Heterogeneous nuclear ribonucleoprotein D0 (hnRNP D0), also known as AU-rich element RNA-binding protein 1 (AUF1), is a well-characterized ARE-binding factor that destabilizes mRNA, while human (Hu) antigen proteins of the ELAV (embryonic lethal, abnormal vision) family are known to stabilize mRNA. AUF1 has four isoforms, p37, p40, p42, and p45, generated by alternative splicing. AUF1 contains two tandem RRMs and an adjacent Q-rich motif. Many proteins regulate mRNA stability by interacting with the AU-rich elements (AREs) in the 3′-untranslated regions (3′-UTRs) of mRNAs.

We obtained the AUF1-p37RRMs protein by RNase treatment and determined the high resolution crystal structure of AUF1-RRM1. A selected AUF1-p37RRMs crystal was diffracted to a resolution of 1.7 Å and belonged to space group P212121. Consequently, we produced selenomethionine-substituted crystals using similar conditions and experimental SAD phasing succeeded using the AutoSol pipeline in the Phenix program. However, after refinement we realized that the two models of RRMs were identical because they had the same sequences as RRM1. The monomeric RRM1 molecule shows a typical RRM structure that contains αβ sandwich with a βαββαβ topology. The PISA analysis, based on the calculated interface area of 374.2 Å2 for the two RRM1 molecules, indicates that the arrangement of RRM1 dimer is most likely generated by crystallographic packing. The two RRM1 molecules are easily superimposed with a root-mean-square deviation (RMSD) of 1.80 Å for 79  Cα, except for the loops β2β3 (L1) and α2β4 (L2). Taken together, these results suggest that the linker between the RRM1 and RRM2 AUF1-p372RRMs proteins was cleaved by a certain protease, possibly a serine protease, and the free RRM1 fragment was specifically crystallized 1 or 2 days later. Although we only obtained the AUF1-RRM1 structure, it is still possible to compare the structure with other tandem RRM structures such as HuR and hnRNP A1, because two molecules of AUF1-RRM1 are found in the asymmetric unit.

> MSKNEEMEGKMFIGGLSWDTTKKDLKDYFSKFGEVVDCTLKLDPITGRSRGFGFVLFKESESVDKVMDQKEHKLNGKVIDPKRAKAM;> MEGKMFIGGLSWDTTKKDLKDYFSKFGEVVDCTLKLDPITGRSRGFGFVLFKESESVDKVMDQKEHKLNGKVIDPKRAKAMA>[4x]MKREEYLKNYLESYLRKKEVSLTEEEFNVI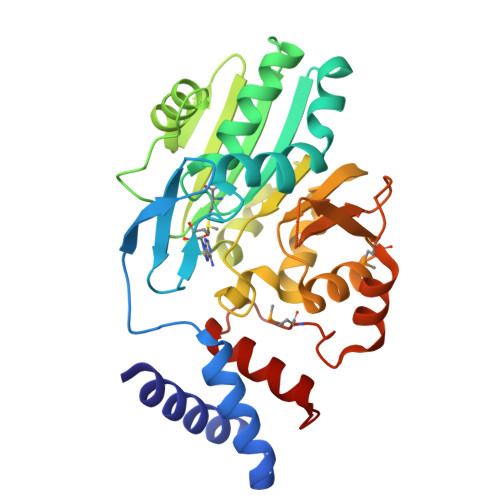LREFLRFAYNPEESGQEIADTADGSKTLIHKTYGEPYHSQTAGAIRESLYKFVRPSRILEKAKERKVIRILDVGFGLGYNLAVALKHLWEVNPKLRVEIISFEKELLKEFPILPEPYREIHEFLLERVPEYEGERLSLKVLLGDARKRIKEVENFKADAVFHDAFSPYKNPELWTLDFLSLIKERIDEKGYWVSYSSSLSVRKSLLTLGFKVGSSREIGRKRKGTVASLKAPVPPMEENEVRKLVLSPFAVPMRDEKLDKEPLEILIDYLLKVYKISR> MGHHHHHHMGQRLLGQKARMVKMYMACRNDIHRYDATFIAIYKSLIPAEEELEKQRQLMAHLENLVAKEWPHAKLYLYGSCANSFGFPKSDIDVCLAIEGDDINKSEMLLKLAEILESDNLQNVQALTRARVPIVKLMDPVTGISCAICINNVLAVVNTKLLRDYAQIDVRLRQLAFIVKHWAKSRRVNETYQGTLSSYAYVLMCIHFLQQRRPPILPCLQEMEPTYS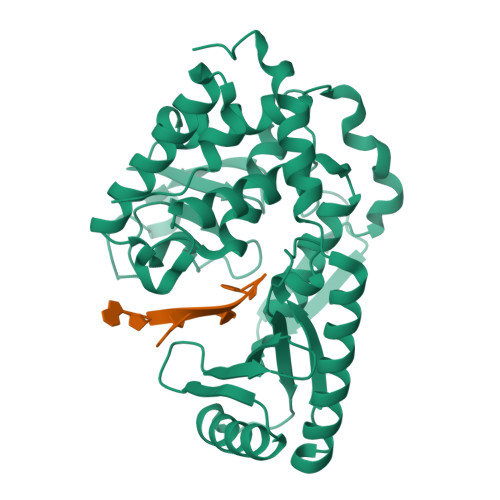VRVDNIRCTYFDNVDRLRNFGSNNRETIAELVWGFFNYWAYAHDYAYNVVSVRTGSILGKREKDWTRRVGNDRHLICIEDPFETSHDLGRVVDKFSIRVLREEFERAARIMHQDPNPCAKLLEPYIPEDNNGQGHN> GTTVTDCTPGPNQNGVTSVQGDEYRVQTN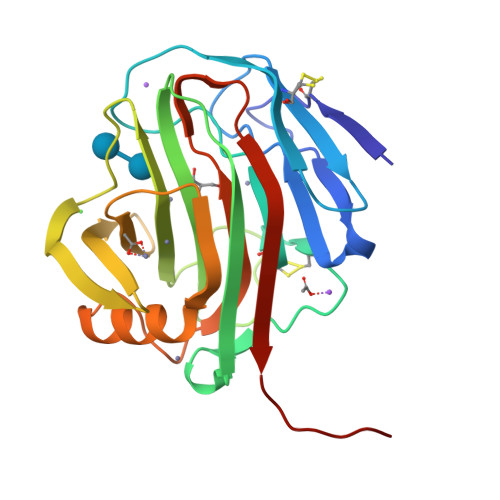EWNSSAQQCLTINTATGAWTVSTANFSGGTGGAPATYPSIYKGCHWGNCTTKNVGMPIQISQIGSAVTSWSTTQVSSGAYDVAYDIWTNSTPTTTGQPNGTEIMIWLNSRGGVQPFGSQTATGVTVAGHTWNVWQGQQTSWKIISYVLTPGATSISNLDLKAIFADAAARGSLNTSDYLLDVEAGFEIWQGGQGLGSNSFSVSVTSGASHHHHHH> GASPSAQELKEQGNRLFVGRKYPEAAACYGRAITRNPLV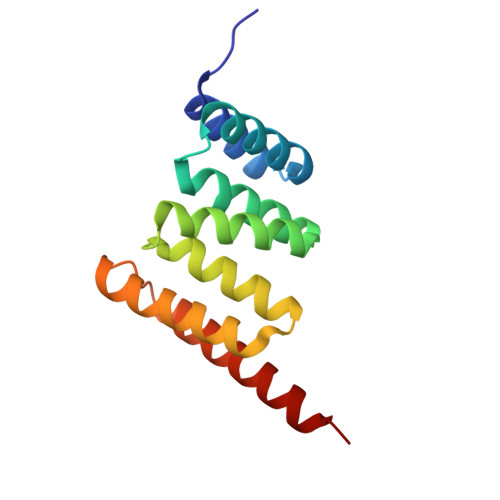AVYYTNRALCYLKMQQHEQALADCRRALELDGQSVKAHFFLGQCQLEMESYDEAIANLQRAYSLAKEQRLNFGDDIPSALRIAKKKRWNSIEERR>MVLYFIGLGLYDERDITVKGLEIAKKCDYVFAEFYTSLMAGTTLGRIQKLIGKEIRVLSREDVELNFENIVLPLAKENDVAFLTPGDPLVATTHAELRIRAKRAGVESYVIHAPSIYSAVGITGLHIYKFGKSATVAYPEGNWFPTSYYDVIKENAERGLHTMLFLDIKAEKRMYMTANEAMELLLKVEDMKKGGVFTDDTLVVVLARAGSLNPTIRAGYVKDLIREDFGDPPHILIVPGKLHIVEA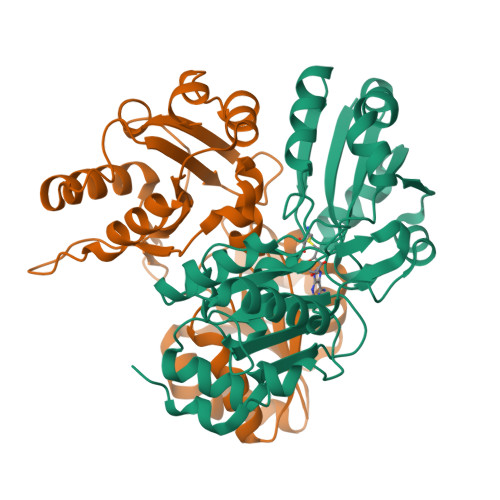EYLVEIAGAPREILRVNV[2x]Here, we report the crystal structure of a SAM-dependent methyltransferase from anammox bacteria (AmxMT1) that has a substrate and active site pocket between a class I SAM methyltransferase-like core domain and an additional α-helix inserted into the core domain. Two SAM-MTs (AmxMT1, 2) are found in many species and genera of anammox bacteria. AmxMT1 is categorized as a class I SAM-MT, which has a Rossmann fold and is the largest family of SAM-MTs, and the enzyme is unusual because it is phylogenetically distant from homologous SAM-MTs in this family. Structural comparisons with homologous SAM-dependent C-methyltransferases in polyketide synthase, AmxACP pull-down assays, AmxACP/AmxMT1 complex structure predictions by AlphaFold, and a substrate docking simulation suggested that a small compound connected to AmxACP could be inserted into the pocket of AmxMT1, and then the enzyme transfers a methyl group from SAM to the substrate to produce branched lipids.

We determined the crystal structure of AmxMT1 by single-wavelength anomalous dispersion (SAD) phasing at 1.60-Å resolution, and one molecule was found in the asymmetric unit. AmxMT1 has an NAD(P)-binding Rossmann fold similar to the αβα sandwich core domain, which consists of seven β-strands and five α-helices and is commonly found in class I SAM-MTs. An α-helix (α9) was inserted between β-strand 7 and α-helix 10 of the core domain. The core domain and α9 are covered by an additional α-domain at the N-terminus, and S-adenosyl-l-homocysteine (SAH) is located in the pocket between the core domain and inserted helix, although we added SAM to the enzyme for crystallization. The ribosyl moiety of the bound SAH forms hydrogen bonds with D202, a water molecule, and the main-chain NH of G182. The terminal carboxyl group of SAH forms a salt bridge with R159 and a hydrogen-bond network that includes a water molecule and several main-chain atoms (carbonyl groups of Y181 and A249; and NH of G184 and F185). The adenine ring is surrounded by aromatic side chains F138, F203, F232, Y254, and W229, and its edge is exposed to the molecular surface. In the crystal structure of AmxMT1, a similar long pocket and SAH were found between the core domain and inserted helix α9. A His-Glu dyad (H304-E308) and Y254 were also found on the surface of the pocket. The substrate binding pocket of AmxMT1 is shorter than that of CurJ C-MT and narrower than that of citrinin synthase CMeT, implying that the substrate of AmxMT1 has a short chain connected to AmxACP3 through the phosphopantetheine group.

> MNQSVDSPNIKLLLSQSHPQMFLTDRLIRFVEEEGISELLQSMRRFTIEEALEAFREKLGYKLQDRVRLRMAKVIVDLLYECEYLEKKGERYFWIEGKGFETKLSADGYKVAKDAFKGQVDFFERCIMYADKFLNGNPPLYSFDSASTGIWEEFLGNTEFRFARSVLINLLFSGRNDNATVLALCYGPGFDILQMQEQYNIRVTALDFKDVFQSQASRRILNPNSVKWVQSALWKGFGTPLPFHDTMFDAVFFACADPYIPEESREFVYKDIFRVLKHGGILGIVTRSYPDTERKYVKDPFVRKGTLCHDFSESVCEGWCGFYHPQESENLFKTIGYHVNTIMLNASVWRLDKP> MKKKPFSILFMGIEDYATKGQKGRSDSLIVVTLDPKNKTMKMLSIPRDTRVQL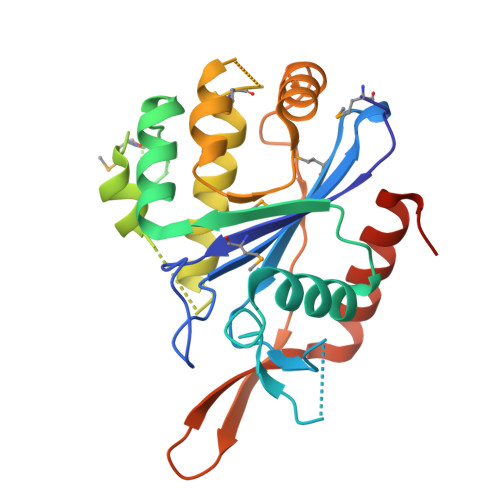AGDTTGSKTKINAAYSKGGKDETVETVENFLQIPIDKYVTVDFDGFKDVINEVGGIDVDVPFDFDEKSDVDESKRIYFKKGEMHLNGEEALAYARMRKQDKRGDFGRNDRQKQILNALIDRMSSASNIAKIDKIAEKASENVETNIRITEGLALQQIYSGFTSKKIDTLSITGSDLYLGPNNTYYFEPDATNLEKVRKTLQEHLDYTPLEHHHHHH>MSHTSTRVAIVTGAAQGLGASIALRLADDGLDVAVNDIGSKSDQLQQIVAQIQAKGRRALAVPADVSRDVDVQAMVAKVVEELGGLDVVRGSPVAAPSTTNLMCYVVYDLQMVANAGIVLYQSLADTQLEVWDRIMSVNLRGVMLCYKYAGVQMIKQGRGGRII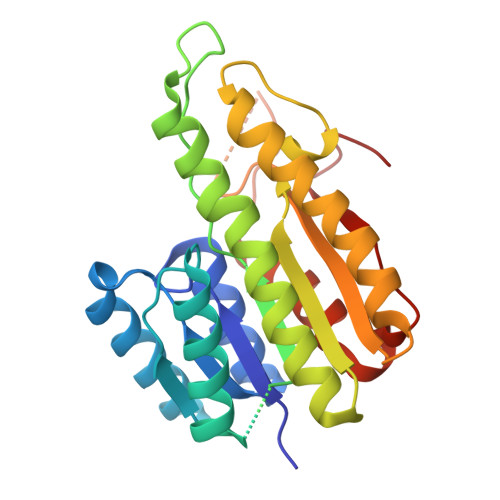AASSAAGKKGMINLPAYSASKFAVRGITQSAALEFAPHNITVNAYCPGGIRTPMSSHADIKLLDLPTNLPFADPEVVASLVSYLAKPEAYFITGQSILVDGGVLFD[8x]> 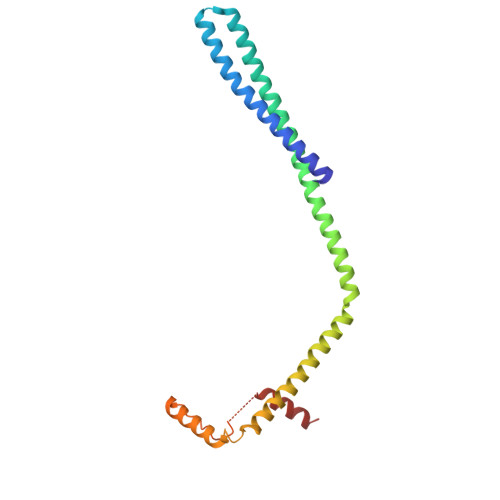MSNMEKHLFNLKFAAKELSRSAKKCDKEEKAEKAKIKKAIQKGNMEVARIHAENAIRQKNQAVNFLRMSARVDAVAARVQTAVTMGKVTKSMAGVVKSMDATLKTMNLEKISALMDKFEHQFETLDVQTQQMEDTVSSTTTLTTPQNQVDMLLQEMADEAGLDLNMELPQGQTGSVGTSVASAEQDELSQRLARLRDQV> MSEKHPGPLVVEGKLTDAERMKHESNYLRGTIAEDLNDGLTGGFKGDNFLLIRFHGMYQQDDRDIRAERAEQKLEPRHAMLLRCRLPGGVITTKQWQAIDKFAGENTIYGSIRLTNRQTFQFHGILKKNVKPVHQMLHSVGLDALATANDMNRNVLCTSNPYESQLHAEAYEWAKKISEHLLPRTRAYAEIWLDQEKVATTDEEPILGQTYLPRKFKTTVVIPPQNDIDLHANDMNFVAIAENGKLVGFNLLVGGGLSIEHGNKKTYARTASEFGYLPLEHTLAVAEAVVTTQRDWGNRTDRKNAKTKYTLERVGVETFKAEVERRAGIKFEPIRPYEFTGRGDRIGWVKGIDDNWHLTLFIENGRILDYPARPLKT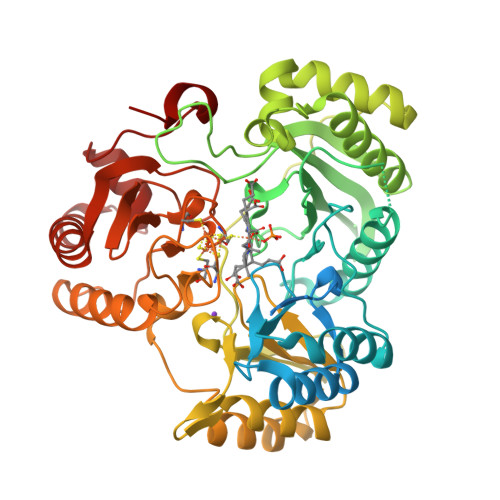GLLEIAKIHKGDFRITANQNLIIAGVPESEKAKIEKIAKESGLMNAVTPQRENSMACVSFPTCPLAMAEAERFLPSFIDNIDNLMAKHGVSDEHIVMRVTGCPNGCGRAMLAEVGLVGKAPGRYNLHLGGNRIGTRIPRMYKENITEPEILASLDELIGRWAKEREAGEGFGDFTVRAGIIRPVLDPARDLWD In living organisms the sulfur atoms needed to synthesize vital sulfur-containing biomolecules, including molybdopterin, biotin, thiamin, the heavily post-translationally modified tRNAs and the ubiquitous Fe-S clusters, are mobilized from L-cysteine as highly reactive persulfidic sulfur atom species by PLP-dependent enzymes known as L-cysteine desulfurases (CDs; E.C. 2.8.1.7). The persulfide moiety is then transferred to desulfurase-specific sulfur acceptor proteins tasked with channeling sulfur down the appropriate pathway to its final destination. The CSD genes, csdA and csdE, encode one CD (CsdA) and one sulfur acceptor (CsdE), which bear a significant degree of sequence similarity to the functionally equivalent SufS and SufE proteins (35% and 45%, respectively) encoded by the SUF system. Unlike SufE, CsdE becomes inactivated in vivo during cell extraction under non-reducing conditions, presumably by disulfide bridge formation through the only cysteine residue in the CsdE protein sequence (Cys61).

In order to shed light into the consequences of oxidation inactivation of the redox-sensitive sulfur acceptor CsdE, we determined the crystal structure of a disulfide-bridged CsdE dimer at 2.4 Å. We used single-wavelength anomalous diffraction at the selenium absorption edge (Se-SAD) to phase selenomethionyl-labeled CsdE crystals that diffracted to 2.95 Å, and performed phase extension in nearly isomorphous native CsdE crystals to 2.4 Å. The final model contains nearly all CsdE residues except for the first 7−8 amino acids, which were disordered. It consists of a two-layered α/β-sandwich with a central three-stranded antiparallel β-sheet (βA-βC), surrounded by seven α-helices (α1-α7); the reactive sulfur acceptor Cys61 is located at the tip of an extended β-hairpin between βA and βB. The disulfide bridge has a favorable stereochemistry and is well defined in electron density maps. In the disulfide-bridged dimer, the two CsdE subunits are related by a pure rotation around an axis running parallel to the CsdE long molecular axis through 141°. The fifth largest interface, at 393 Å2 or merely 5.4% of a monomer’s ASA, includes the disulfide bond that creates this inactive CsdE species. However, in the disulfide-bridged CsdE structure this secluded orientation is obviously not possible; instead, the loop containing Cys61 has turned around to expose the thiol sulfur atom for disulfide bond formation. Indeed, the dimeric Cys61 conformation is roughly halfway between the fully protected and the completely exposed conformations, thereby representing an intermediate state. A remarkable observation made in the CsdE dimer is that, while Cys61 presents a fully exposed state as in persulfurated (CsdA-CadE), helix α7 is essentially unchanged with respect to the free forms of CsdE, and it is only slightly tilted to make way for the outward-going Cys61 loop.

>MTNPQFAGHPFGTTVTAETLRNTFAPLTQWEDKYRQLIMLGKQLPALPDELKAQAKEIAGCENRVWLGYTVAENGKMHFFGDSEGRIVRGLLAVLLTAVEGKTAAELQAQSPLALFDELGLRAQLSASRSQGLNALSEAIIAATKQVKHHHHHH[2x]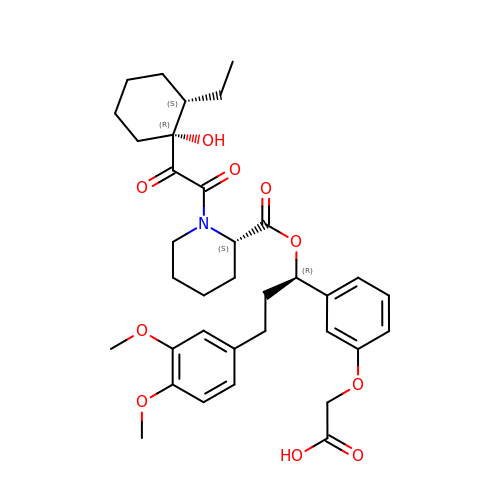{3-[(1R)-3-(3,4-dimethoxyphenyl)-1-({[(2S)-1-{[(1R,2S)-2-ethyl-1-hydroxycyclohexyl](oxo)acetyl}piperidin-2-yl]carbonyl}oxy)propyl]phenoxy}acetic acid | C35 H45 N O10 | JLRDMSUQFUWACS-RORDBKJESA-N> PCYTATRSECKQKHKFVPGVWMAGEGMDVTTLRRSGSFPVNTQRFLRPDRTCTLCKN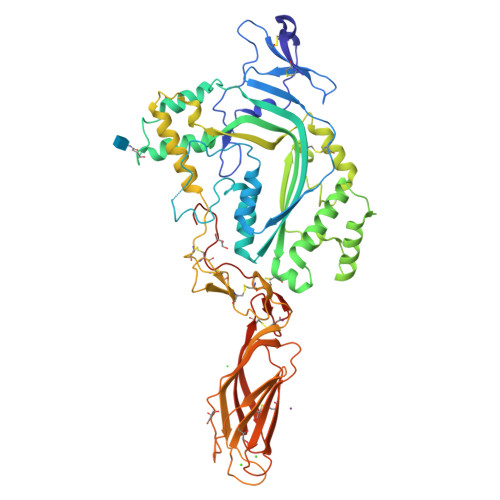SLMRDATQRLPVAITHWRPHSSHCQRNVAAAKVHSTEGVAREAAANINNDWRVGLDVNPRPEANMRASVAGSHSKVANFAAEKTYQDQYNFNSDTVECRMYSFRLVQKPPLHLDFKKALRALPRNFNSSTEHAYHELISSYGTHFITAVDLGGRISVLTALRTCQLTLNGLTADEVGDCLNVEAQVSIGAQASVSSEYKACEEKKKQHKMATSFHQTYRERHVEVLGGPLDSTHDLLFGNQATPEQFSTWTASLPSNPGLVDYSLEPLHTLLEEQNPKREALRQAISHYIMSRARWQNCSRPCRSGQHKSSHDSCQCECQDSKVTNQDCCPRQRGLAHLVVSNFRAEHLWGDYTTATDAYLKVFFGGQEFRTGVVWNNNNPRWTDKMDFENVLLSTGGPLRVQVWDADYGWDDDLLGSCDRSPHSGFHEVTCELNHGRVKFSYHAKCLPHLTGGTCLEYAPQGLLGDPPGNRSGAVWHHHHHH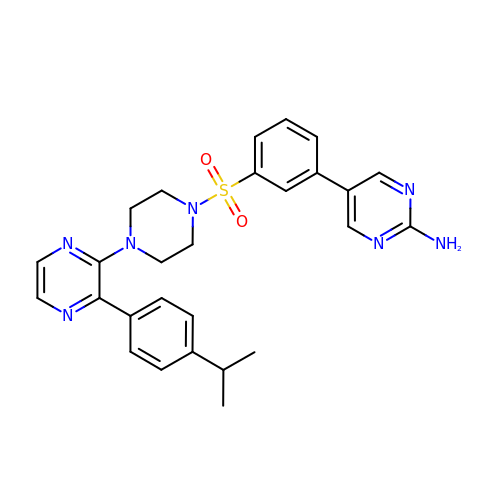5-{3-[(4-{3-[4-(1-methylethyl)phenyl]pyrazin-2-yl}piperazin-1-yl)sulfonyl]phenyl}pyrimidin-2-amine | C27 H29 N7 O2 S | IVXKQJAJTVBVLV-UHFFFAOYSA-N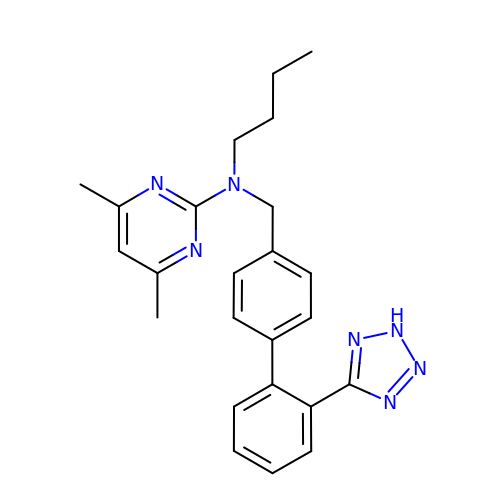N-butyl-4,6-dimethyl-N-{[2'-(2H-tetrazol-5-yl)biphenyl-4-yl]methyl}pyrimidin-2-amine | C24 H27 N7 | ZSQBWJVNWXAGKO-UHFFFAOYSA-N>[3x]GSMKGSRIELGDVTPHNIKQLKRLNQVIFPVSYNDKFYKDVLEVGELAKLAYFNDIAVGAVCCRVDHSQNQKRLYIMTLGCLAPYR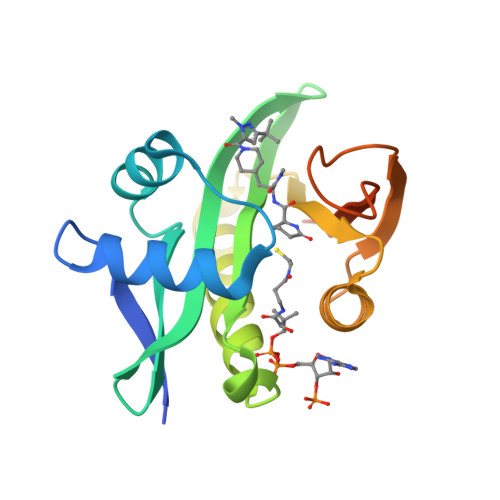RLGIGTKMLNHVLNICEKDGTFDNIYLHVQISNESAIDFYRKFGFEIIETKKNYYKRIEPADAHVLQKNLKVPSGQNADVQKTDN>[6x]GMNIVSQLSPVTLSPE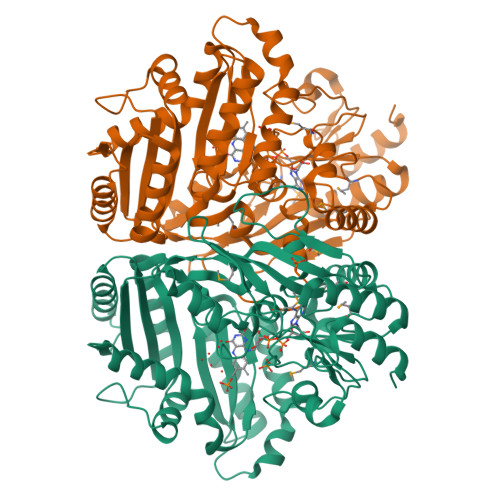LIARFTAIVGDKHALTDPLELEAYITEERNLYRGHSPLVLRPGSTEEVVAICKLANEARVALVPQGGNTGLVGGQTPHNGEVVISLKRMDKIREIDTSSNTITVEAGAILQRVQEKAAEVDRLFPLSLGAQGSCTIGGNLSTNAGGTAALAYGLARDMALGVEVVLADGRVMNLLSKLKKDNTGYDLRDLFIGAEGTLGIITAATLKLFPKPRAVETAFVGLQSPDDALKLLGIAQGEAAGNLTSFELIAETPLDFSVRHANNRDPLEARYPWYVLIELSSPRDDARAALESILERGFEDGIVVDAAIANSVQQQQAFWKLREEISPAQKPEGGSIKHDISVPVAAVPQFIEQANAAVVALIPGARPVPFGHLGDGNIHYNVSQPVGADKAEFLARWHDVSQVVFEVVLRLGGSISAEHGIGVMKRDELAEVKDKTAIELMRSIKALLDPHGIMNPGKVV>[6x]MQIDAVKCATASRNTFNFMIKNIIPNKSIILMKKVYELTSEEALSYFLRHDSYTTLELPAYINFTTLLNDIN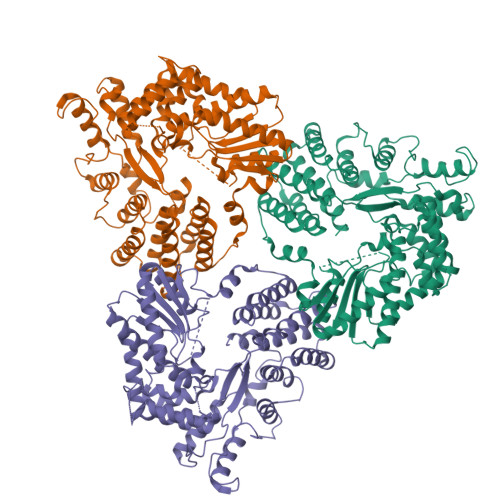SSIHNKKIKIEPTAKELMGKDINYEVLVSKDGLYSWRRITLINPLYYVYFCRKITAPATWEIITEKFKSFESNDLFTCSSIPVRKDNSSNIAASVMNWWEDFEQKSLALALEYEFMFSTDISNFYPSIYTHSFEWVFISKEEAKKKKSKNNPGGLIDSHIQMMMNNQTNGIPLGSTLMDTFAELILGQIDIELRKKTNELKIINYKVVRYRDDYRIFSNSKDDLDIISKCLVNVLGDFGLDLNSKKTELYEDIILHSLKQAKKDYIKEKRHKSLQKMLYSIYLFSLKHPNSKTTVRYLNDFLRNLFKRKTIKDNGQQVDAMLGIISSIMAKNPTTYPVGTAIFSKLLSFLYGDDTQKKLTKLEQLHKKLDKQPNTEMLDIWFQRTQAKINLEWNKSYKSALCVRINDELTKEKTFSVNNLWNIDWIQGKETSPNKAKILSLLRKTKIVDTDKFDKMDDNITPEEVNLFF>CPRFLKVKNWETDVVLTDTLHLKSTLETGCTEHICMGSIMLPSQHTRKPEDVRTKDQLFPLAKEFLDQYYSSIKRFGSKAHMDRLEEVNKEIESTSTYQLKDTELIYGAKHAWRNASRCVGRIQWSKLQVFDARDCTTAHGMFNYICNHVKYATNKGNLRSAITIFPQRTDGKHDFRVWNSQLIRYAGYKQPDGSTLGDPANVQFTEICIQQGWKAPRGRFDVLPLLLQANGNDPELFQI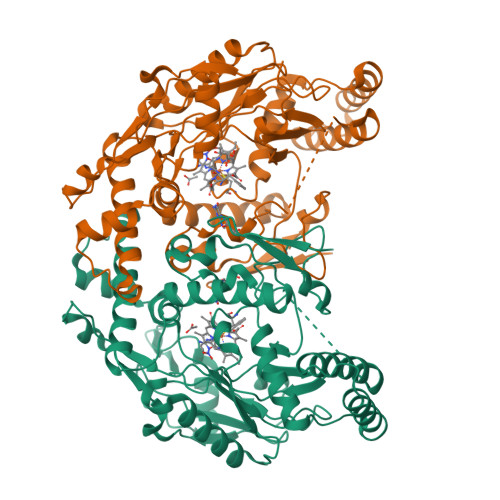PPELVLEVPIRHPKFDWFKDLGLKWYGLPAVSNMLLEIGGLEFSACPFSGWYMGTEIGVRDYCDNSRYNILEEVAKKMDLDMRKTSSLWKDQALVEINIAVLYSFQSDKVTIVDHHSATESFIKHMENEYRCRGGCPADWVWIVPPMSGSITPVFHQEMLNYRLTPSFEYQPDPWNTHVWK[2x]> DCLSGWSSYEGHCYKAFEKYKTWEDAERVCTEQAKGAHLVSIESSGEADFVAQLVTQNMKRLDFYIWIGLRVQGKVKQCNSEWSDGSSVSYENWIE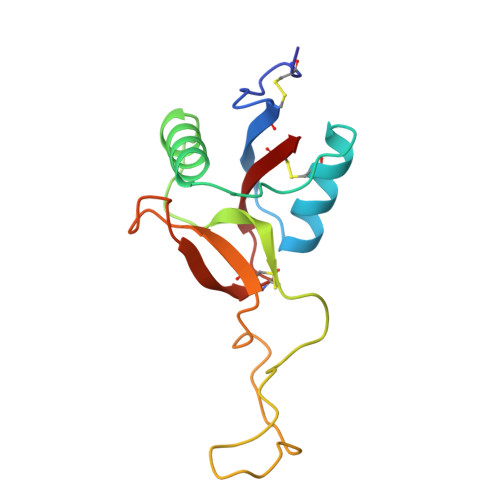AESKTCLGLEKETDFRKWVNIYCGQQNPFVCEA>[2x]MGGFFARLKRSLLKTKENLGSGFISLFRGKKIDDDLFEELEEQLLIADVGVETTRKIITNLTEGASRKQLRDAEALYGLLKEEMGEILAKVDEPLNVEGKTPFVILMVGVNGVGKTTTIGKLARQFEQQGKSVMLAAGDTFRAAAVEQLQVWGQRNNIPVIAQHTGADSASVIFDAIQAAKARNIDVLIADTAGRLQNKSHLMEELKKIVRVMKKLDVEAPHEVMLTIDASTGQNAVSQAKLFHEAVGLTGITLTKLDGTAKGGVIFSVADQFGIPIRYIGVGERIEDLRPFKADDFIEALFAREDHHHHHH

The stringent response enables bacteria to respond to nutrient limitation and other stress conditions through production of the nucleotide-based second messengers ppGpp and pppGpp, collectively known as (p)ppGpp. Here, we report that (p)ppGpp inhibits the signal recognition particle (SRP)-dependent protein targeting pathway, which is essential for membrane protein biogenesis and protein secretion. More specifically, (p)ppGpp binds to the SRP GTPases Ffh and FtsY, and inhibits the formation of the SRP receptor-targeting complex, which is central for the coordinated binding of the translating ribosome to the SecYEG translocon. Briefly, SRP recognizes hydrophobic signal sequences in the context of translating ribosomes, and SRP bound to ribosome-nascent chain complexes (RNCs) in turn interacts in a GTP-dependent manner with its receptor FtsY, also a GTPase, which localizes at the cytoplasmic membrane periphery of bacteria via a membrane-targeting sequence.

For the NG domain of the SRP-receptor (Ec)FtsY a KD of 21.7 ± 5.4 µM for ppGpp and 9.8 ± 1.1 µM for GDP were obtained. We determined the crystal structures of the pppGpp-bound NG domains of (Ec)Ffh and (Ec)FtsY at resolutions of 2.5 and 2.4 Å, respectively, as well as the crystal structures of (Bs)Ffh and (Ec)Ffh in complex with ppGpp and Mg2+ at resolutions of 2.5 and 2.8 Å, respectively. The ppGpp or pppGpp molecules are bound to the G domains of Ffh and FtsY and occupy the canonical guanosine nucleotide-binding site. In detail, the guanine moiety of (p)ppGpp is recognized by the well-described aspartate of the G4 element responsible for the discrimination of guanosine nucleotides by P-loop type GTPases. The α-, β-, and γ-phosphates of (p)ppGpp are coordinated by the G1-element (P-loop), and by residues originating from the switch I and II regions including the G2 and G3 elements, respectively. The δ- and ε-phosphate, which are covalently bound to the 3′-OH group of the ribose moiety and discriminate (p)ppGpp from its GDP/GTP counterparts, point away from the active sites of both GTPases. Both phosphates are not coordinated or form any obvious contacts to the GTPases of Ffh and FtsY. Our structural analysis of (p)ppGpp-bound Ffh or FtsY now shows that this reciprocal nucleotide arrangement is no longer possible, when the δ-, ε-pyrophosphate moieties at the 3′-OH group of the alarmones prevent the formation of the crucial hydrogen bond, and by introducing electrostatic repulsion by the negatively charged phosphates.>[2x]MFNRLFRVCFLAALIMAFTL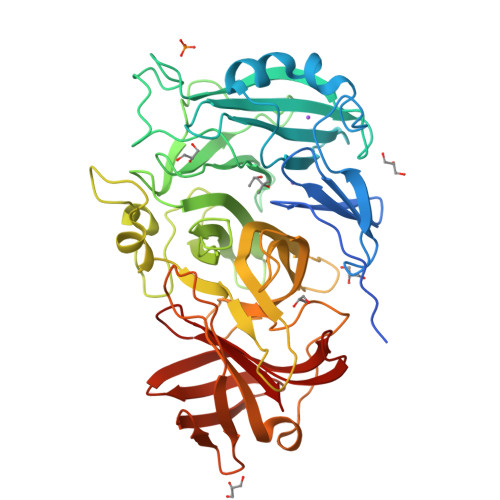PNSVYAQKPIFKEVSVHDPSIIETNGTFYVFGSHLASAKSNDLMQWQQLTTSVSNDNPLIPNVYEELKETFEWAQSDTLWAADVTQLADGKYYMYYNACRGDSPRSAMGVAVADNIEGPYKNKGIFLKSGMEGTSSDGTPYDATKHPNVVDPHTFFDKDGKLWMVYGSYSGGIFILEMNPKTGFPLPGQGYGKKLLGGNHSRIEGPYVLYNPDTQYYYLYLSYGGLDATGGYNIRVARSKKPDGPYYDAEGNPMLDVRGKGGTFFDDRSIEPYGVKLMGSYTFETENEKGTGYVSPGHNSAYYDEKTGRSYLIFHTRFPGRGEEHEVRVHQLFMNKDGWPVAAPYRYAGETLKEVKQKDITGTYKLIQHGKDISADIKQTINIQLNKNHTISGEMTGTWRKTGKNTADITLAGKKYNGVFLRQWDSVREKNVMTFSVLNTSGEAVWGSKA> AQPAARDLKVVTKRGSADGCTDWSVDIKKYQVLVGEPVRIKCALFYGYIRTNYSLAQSAGLSLMWYKSSGPGDFEEPIAFDGSRMSKEEDSIWFRPTLLQDSGLYACVIRNSTYCMKVSISLTVGENDTGLCYNSKMKYFEKAELSKSKEISCRDIEDFLLPTREPEILWYKECRTKAWRPSI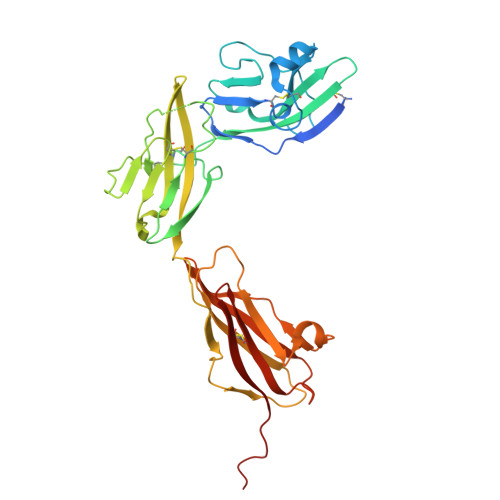VFKRDTLLIKEVKEDDIGNYTCELKYGGFVVRRTTELTVTAPLTDKPPKLLYPMESKLTVQETQLGGSANLTCRAFFGYSGDVSPLIYWMKGEKFIEDLDENRVWESDIRILKEHLGEQEVSISLIVDSVEEGDLGNYSCYVENGNGRRHASVLLHKRKHHHHHH> PAQDNSRFVIRDRNWHPKALTPDYKTSIARSPRQALVSIPQSISETTG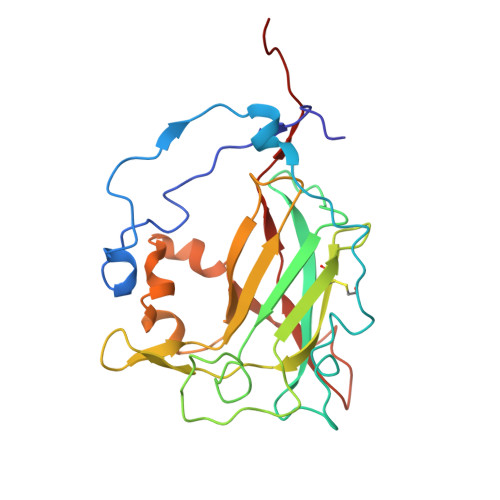PNFSHLGFGAHDHDLLLNFNNGGLPIGERIIVAGRVVDQYGKPVPNTLVEMWQANAGGRERHKNDRYLAPLDPNFGGVGRCLTDSDGYYSFRTIKPGPYPWRNGPNDWRPAHIHFGISGPSIATKLITQLYFEGDPLIPMCPIVKSIANPEAVQQLIAKLDMNNANPMDCLAYRFDIVLRGQRKTHFENC> MDYKDDDDKNRALSPMVSEFETIEQENSYNEWLRAKVATSLADP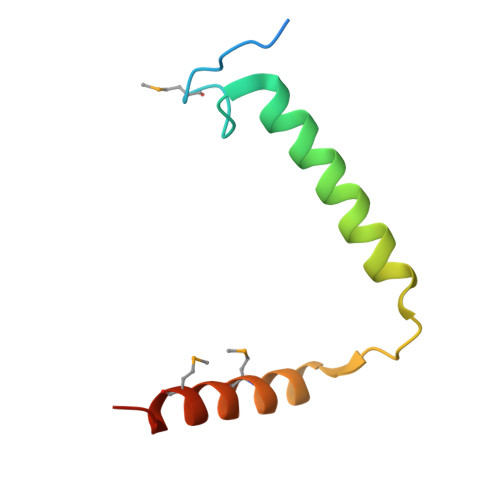RPAIPHDEVERRMAERFAKMRKERSKQ> QGMDFLTSTLLSGILYDGFKNGVAITTGFLKEKLHGWIVDDTLLETLAYKVNTLELKDYGEHVIERKLNESSEIQQILKLIQPEQ;>MDFLTSTLLSGILYDGFKNGVAITTGFLKEKLHGWIVDDTLLETLAYKVNTLELKDYGEHVIERKLNESSEIQQILKLIQPE[2x];> MDFLTSTLLSGILYDGFKNGVAITTGFLKEKLHGWIVDDTLLETLAYKVNTLELKDYGEHVIERKLNESSEIQQILKLIQPEQN;> GMDFLTSTLLS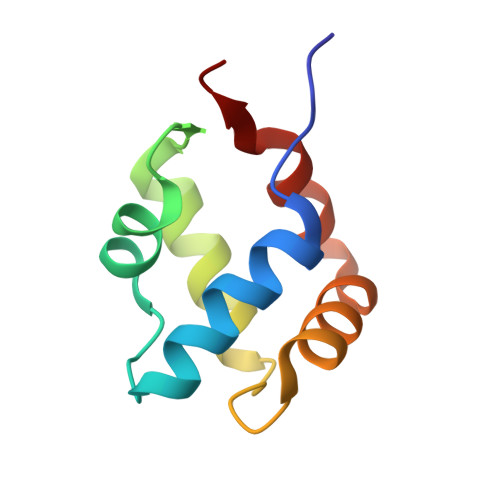GILYDGFKNGVAITTGFLKEKLHGWIVDDTLLETLAYKVNTLELKDYGEHVIERKLNESSEIQQILKLIQPEQN;>[2x]GMDFLTSTLLSGILYDGFKNGVAITTGFLKEKLHGWIVDDTLLETLAYKVNTLELKDYGEHVIERKLNESSEIQQILKLIQPE;> GMDFLTSTLLSGILYDGFKNGVAITTGFLKEKLHGWIVDDTLLETLAYKVNTLELKDYGEHVIERKLNESSEIQQILKLIQPEQ>[3x]ETAAAPYPLAHPPRLADYLPPPPAADSAAAVADLGAVLEAQRLRTPEQVRRVRAHDHPEDNVFPFAGDLLGASFDKERLPLTRSFFNRAQ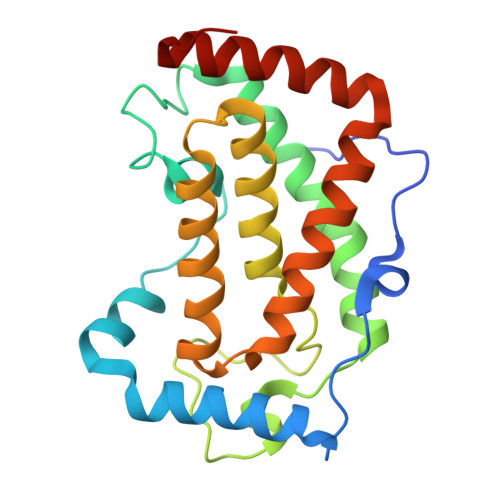ENLVEVLMPAKKHFARPRPYEVTPKVKPVLPPPEGESYPSGHTMRSYFKASLLSMLVPEHHDAFFARAEEHAQSRVLAGVHFPSDLEGGQTAAAALVASLLADPAVAADFAAVREELRGALGLPKLQ>HMPVQPIKLYYLPPSPPCR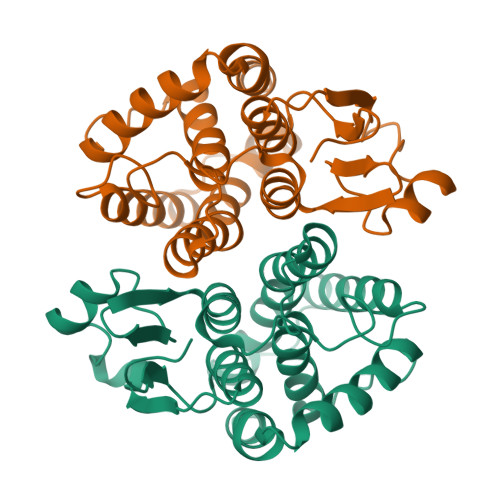AVMMTARVLELDLHLITTNIMNGEHMTPEYLKMNPQHTIPTMDDNGFILWESRAIQTYLVNAYGKDDSLYPKNPRQRAIIDQRLNFDLGTLYLRYLNLYTPILFRGEAYDQEKADKFDEALGWLNTFLDGRPFVAGENMTVADITIVVTITNIDAFGYDFSSHENIAKWFERTKKMLEPYGYDEIDVTGAKMLASFLKKE[4x]> VDCSEYPKPACTXDYRPLCGSDNKTYGNKC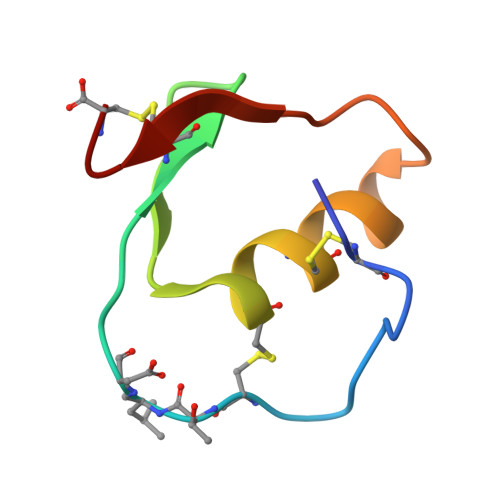NFCNAVVESNGTLTLSHFGKC>MAFKVISQENLLEQKRKETLQEDIPFIVNGEMEYVTKKISNGEMETLELNKPLGEMMTFSSTSNLKELLRKVVLDVELGREQVQLLYKPIYDSIADSNLPQVMDAKWALQGNCVFLEHIEGEEIKFGTINAENGPVARIQTYATGFEYTKEMKDFNQTFSVEILNKSIGESYNALLNHIHLSPIINFNYKASNKTAFKGETNDPIWLGIWRTLTQAQKDTVIAKRQGNILMASSADQIEIEMALNGGHLLNGSMYPSIKNISTVIYYDGWEVTVGKKTYSYKGVTPGKGYLIRPKRGFKELIKRDLTTE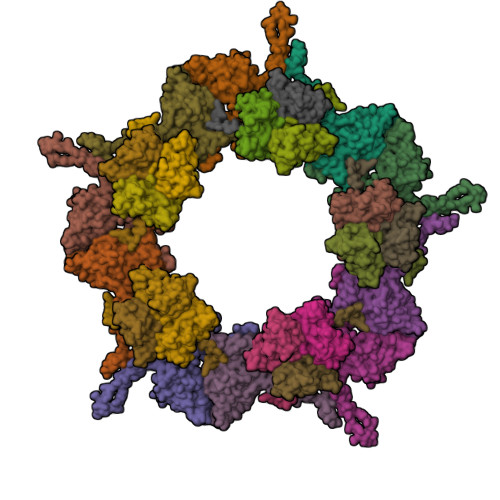VGNADLSKLVENQIVGHCYRGAFAAVEENVQEISFR[10x];>MAFKGQPTPSTITQITRAKISDGKSVRVILSEGESTKTQQFYLINGFFGVAMQDGEKGDEVTLQIEQAEYETDNIVTSEAFEAGKLIYWDNTAKKFTTTSASNRLVGRVTDGKDSNNVIWFILLPQQ[15x]>MGSSHHHHHHSSGLVPRGSHSDEVDAHMTTNTVSRKVAWLRVVTLAVAAFIFNTTEFVPVGLLSDIAQSFHMQTAQVGIMLTIYAWVVALMSLPFMLMTSQVERRKLLICLFVVFIASHVLSFLSWSFTVLVISRIGVAFAAAIFWSITASLAIRMAPAGKRAQALSLIATGTALAMVLGLPLGRIVGQYFGWRMTFFAIGIGALITLLCLIKLLPLLPSEHSGSLKSLPLLFRRPALMSIYLLTVVVVTAHYTAYSYIEPFVQNIAGFSANFATALLLLLGGAGIIGSVIFGKLGNQYASALVSTAIALLLVCLALLLPAANSEI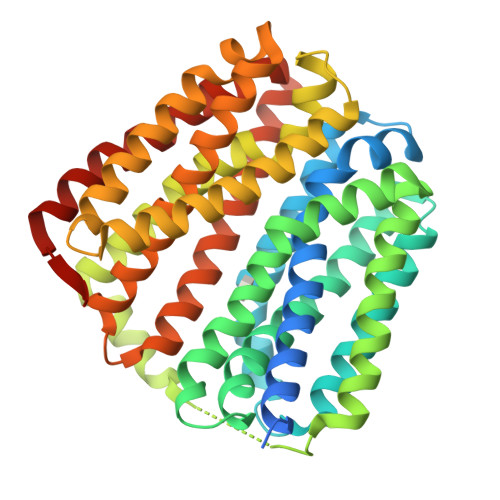HLGVLSIFWGIAMMIIGLGMQVKVLALAPDATDVAMALFSGIFNIGIGAGALVGNQVSLHWSMSMIGYVGAVPAFAALIWSIIIFRRWPVTLEEQTQ[3x]> NDPITNAVESAVSALADTTISRVTAANTAASTHSLGTGR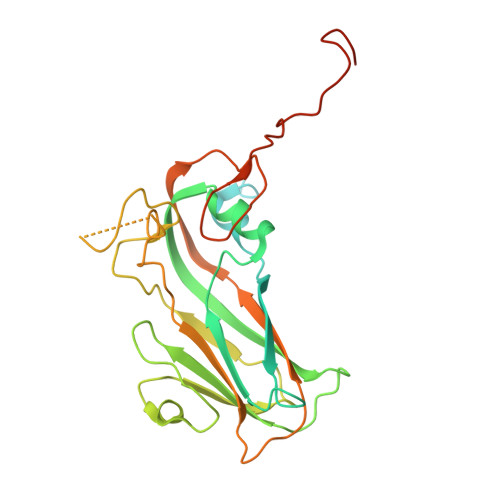VPALQAAETGASSNSSDENLIETRCVMNRNGVNEASVEHFYSRAGLVGVVEVKDSGTSLDGYTVWPIDVMGFVQQRRKLELSTYMRFDAEFTFVSNLNNSTTPGMLLQYMYVPPGAPKPDSRKSYQWQTATNPSVFAKLSDPPPQVSVPFMSPATAYQWFYDGYPTFGEHKQATNLQYGQCPNNMMGHFAIRTVSESTTGKNIHVRVYMRIKHVRAWVPRPLRSQAYMVKNYPTYSQTITNTATDRASITTTDYEGGVPASPQRTS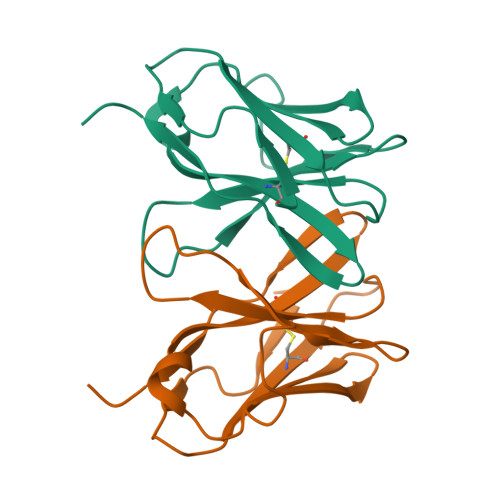>[2x]MPSPFRLSPVRVEGRLGQRVELQCEVLLSSAAPGCTWLFQKNEPAARPIFLAYLSRSRTKLAEELDPKQISGQRIQDTLYSLTLHRFRKEEEGYYFCSVVSNSVLYFSAFVPVFLPVKPTTTP The Mex67–Mtr2 complex (NXF1–NXT1 in metazoans and small bristles in Drosophila melanogastor) is the principal mRNA-export factor in Sacccharomyces cerevisiae. Mex67/NXF1 is a modular protein constructed from four domains: an RNA-recognition motif (RRM) domain, a leucine-rich repeat (LRR) domain, a nuclear transport factor 2-like (NTF2L) domain and an ubiquitin-associated (UBA) domain. Mtr2 is a ∼15–20 kDa protein that also has an NTF2-like fold and forms a tight heterodimeric complex with the Mex67 NTF2L domain.

An unexpected homodimeric form of ctMex67 was also observed in which the two copies of ctMex67NTF2L formed a dimer analogous to that in S. cerevisiae NTF2. Two copies of the LRR domain were also present in the asymmetric unit, but the LRR-NTF2L linker was disordered. However, the previously ordered pre-α1 loop that gave rise to the asymmetry in the NTF2L–Mtr2 region was now disordered, perhaps thereby allowing the symmetric homodimeric Mex67 to be generated. Moreover, ctMex67LRR-NTF2L appeared to form a homodimer in solution, and in size-exclusion chromatography coupled with multi-angle light scattering the protein migrated as a single peak with a molecular mass of 82 g mol−1, consistent with a dimer (each chain has a theoretical mass of 42 g mol−1). The homodimeric complex of NTF2L domains in the ctMex67LRR-NTF2L crystals was unanticipated because it had been thought that complex formation between Mex67 and Mtr2 was a prerequisite for efficient nuclear export of mRNA. Although SEC-MALS indicated that ctMex67LRR-NTF2L is homodimeric in solution, whether Mex67 is ever not complexed to Mtr2 in vivo is currently unclear and whether the configuration observed simply represents an inactive form of the Mex67–Mtr2 complex or whether homodimeric Mex67 has another role in the cell has yet to be established.

>SMPALSSQSKLSQAAQETKQKLTSCLARRYNAEQKLLDLSALGTDETLSSLGSFNNQSLAEKSFKALMHLVSNEYKDPEQKNEAIQAVSLARNDILDVGQVYSLAVTLPRLRRLDLSGNNLENLSKISKWQQEFRFLEELHLTGNPVTTLPNYATEIKKWFPSLQILDGQQIRTPQEAAESLKSSFPTPLPQLPSNVRDGENNVASTFLQAFFQLWDHDRLTLIPQFYDSETTFSVVFATDSPQDPASSSCSKFSRNLNILSPRHPSTLQRLFVGSNLIADLWKVLPATRHPSLDQTSQWLIDCHTFPHLADPTGMAPYAMGLMINVNGQCEEADISQNLYGTRTFSRCFILGPSKPGAPHPYRVLSDQLTLHTWKPQPAPQVGTV[4x]> GSMPAANSMAMKRETLNLRIKPAERDLIDRAAKARGKNRTDFVLEAARAAAEEALIEQRIIMADPEAYQEFL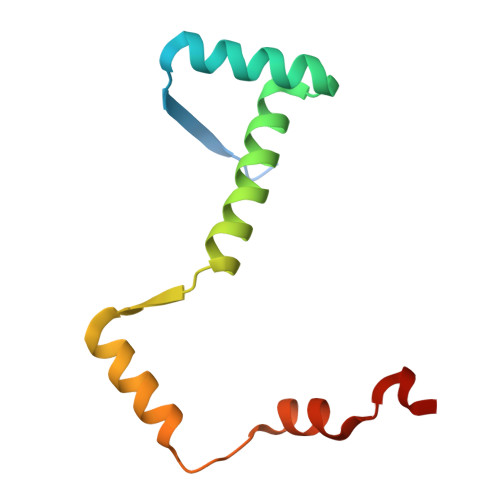VRLDQTPSPNAALRKTMQTPAPWEQEK> GPMGNGMNKILPGLYIGNFKDARDAEQLSKNKVTHILSVHDSARPMLEGVKYLCIPAADSPSQNLTRHFKESIKFIHECRLRGESCLVHSLAGVARSVTLVIAYIMTVTDFGWEDALHTVRAGRSCANPNVGFQRQLQEFEKHEVHQYRQWLKEEYG

DUSP22 is a small phosphatase containing 184 residues, and the sequence contains a catalytic domain as well as an N-terminal myristoylation site. This enzyme is broadly expressed in different tissues and plays important roles in the regulation of signaling pathways, such as inactivating the T cell receptor (TCR) signaling pathway, activating the JNK signaling pathway, and regulating the phosphorylation of focal adhesion kinase (FAK). The phosphatase domain of DUSP22 consists of five twisted β-sheets and six α-helices, and the structural scaffold is similar to that of DUSP3 (VHR), while DUSP22 does not contain an N-terminal α-helix surrounded by the N-loop. In this region, the catalytic activity is facilitated by C88 in the P-loop and D57 in the D-loop, and the hydrogen bonding network is formed by D57 in the D-loop, S93 in the P-loop, and N128 in the N-loop.

The S93 mutants were combined with a second mutation, C88S, to produce proteins for growing better crystals, which improved the resolution (<1.6 Å) and helped to determine the structures. In the crystal structure of C88S/S93A, the overall structure was similar to that of C88S, and the side chains of D57 and N128 also formed a hydrogen bond. A water-mediated hydrogen bonding network was formed among the side chains of D57 and N128, as well as the backbone amide of N128. The position of this water molecule was above the original position of S93 and it did not form a hydrogen bond with the P-loop. A93 in the structure was independent of the water-mediated hydrogen bonding network, and the comparison of B-factor between C88S and C88S/S93A showed that the positional disorder increased on the three loops. The S93A mutation probably resulted in the unstable active site structure and decreased the catalytic efficiency. In the crystal structure, the S93A mutant shows that the P-loop is independent from the interaction of the hydrogen bonding network and the B-factor is increase in the three loops, suggesting that the conformation of the D-loop, P-loop, and N-loop cannot be stabilized. Consistently, the decrease in kcat is observed in the S93A mutant because D57 cannot form a stable interaction with S93.> GASVADKAD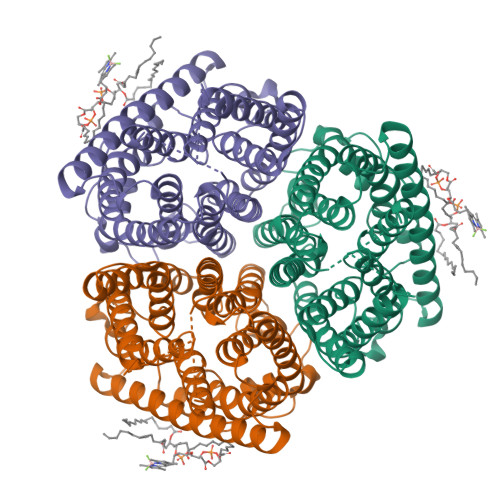NAFMMICTALVLFMTIPGIALFYGGLIRGKNVLSMLTQVTVTFALVCILWVVYGYSLAFGEGNNFFGNINWLMLKNIELTAVMGSIYQYIHVAFQGSFACITVGLIVGALAERIRFSAVLIFVVVWLTLSYIPIAHMVWGGGLLASHGALDFAGGTVVHINAAIAGLVGAYLIGKRVGFGKEAFKPHNLPMVFTGTAILYIGWFGFNAGSAGTANEIAALAFVNTVVATAAAILGWIFGEWALRGKPSLLGACSGAIAGLVGVTPACGYIGVGGALIIGVVAGLAGLWGVTMLKRLLRVDDPCDVFGVHGVCGIVGCIMTGIFAASSLGGVGFAEGVTMGHQLLVQLESIAITIVWSGVVAFIGYKLADLTVGLRVPEEQEREGLDVNSHGENAYNA> MEHKAPLVEFLGLTFNLSDMLMITITCLIVFIIAVAATRSLQLRPTGMQNFMEWVFDFVRGIINSTMDWQTGGRFLTLGVTLIMYVFVANMLGLPFSVHVNGELWWKSPTADATVTLTLAVMVVALTHYYGVKMKGASDYLRDYTR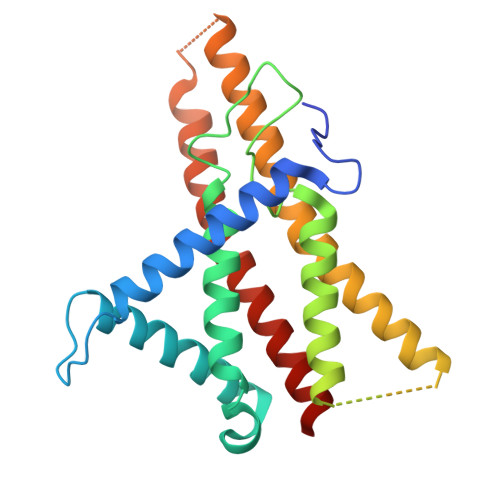PVAWLFPLKIIEEFANTLTLGLRLFGNIYAGEILLGLLASLGTHYGVLGAVGAAIPMMVWQAFSIFVGTIQAFIFTMLTMVYMAHKVSHDH>GQPNSFTNQCPGETCVIPN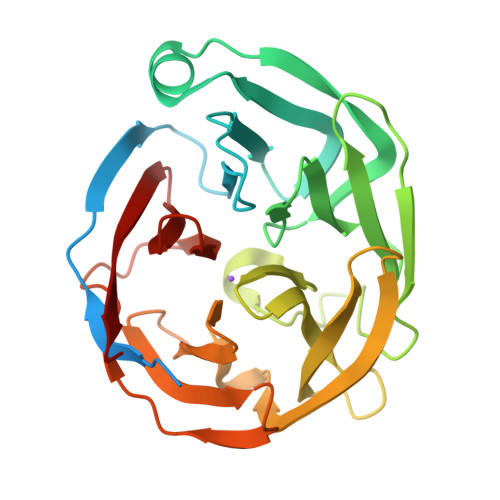DDTLVGRADEKVNERHSPQTEPMITSIGNPAQVLKVKETFGTWLRESANRSDDRIWVTEHFSGIMVKEFEDLPALLNSSFTLLHLPHYFHGCGHAVYNNSLYYHKGGSNTIVRFEFGKETPQTLKLEDALYFDRKYLFANSKTYFNIAVDEKGLWIIYASSVDGSSILVAQLDERTFSVLRHINTTYPKSKAGNAFIAQGILYVTDTKDTRVTFAFDLLRGKQINANFGLRMSQSVLAMLSYNMRDQHLYSWEDGHLMLYPVHFSS[2x]>PIATPYPVKEWLQPKRYKAHLMGTTYVYDFPELFRQASSSQWKNFSADVKLTDDFFISNELIEDENGELTEVEREPGANAIGMVAFKITVKTPEYPRGRQFVVVANDITFKIGSFGPQEDEFFNKVTEYARKRGIPRIYLAANSGARIGMAEEIVPLFQVAWNDAANPDKGFQYLYLTSEGMETLKKFDKENSVLTERTVINGEERFVIKTIIGSEDGLGVECLRGSGLIAGATSRAYHDIFTITLVTCRSVGIGAYLVRLGQRAIQVEGQPIILTGAPAINKMLGREVYTSNLQLGGTQIMYNNGVSHLTAVDDLAGVEKIVEWMSYVPAKRNMPVPILETKDTWDRPVDFTPTNDETYDVRWMIEGRETESGFEYGLFDKGSFFETLSGW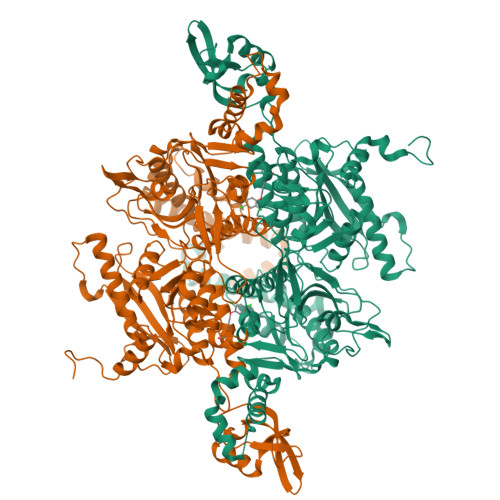AKGVVVGRARLGGIPLGVIGVETRTVENLIPADPANPNSAETLIQEPGQVWHPNSAFKTAQAINDFNNGEQLPMMILANWRGFSGGQRDMFNEVLKYGSFIVDALVDYKQPIIIYIPPTGELRGGSWVVVDPTINADQMEMYADVNARAGVLEPQGMVGIKFRREKLLDTMNRLDDKYRELRSQLSNKSLAPEVHQQISKQLADRERELLPIYGQISLQFADLHDRSSRMVAKGVISKELEWTEARRFFFWRLRRRLNEEYLIKRLSHQVGEASRLEKIARIRSWYPASVDHEDDRQVATWIEENYKTLDDKLKGLKLESFAQDLAKKIRSDHDNAIDGLSEVIK[2x]> MSENQNEKVYDLSFFMPGQTI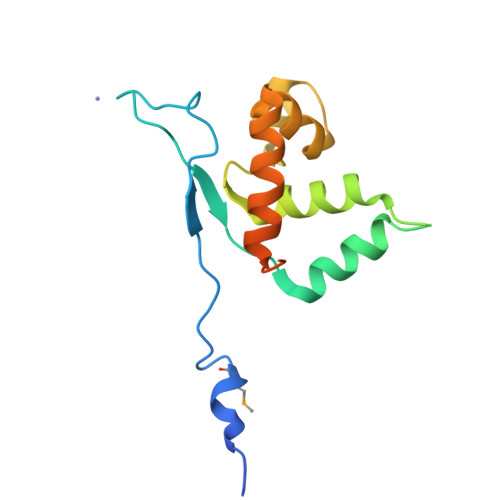DAEEVEVPISKRFVDKEGNVVPFIFKAITTDRIDELEKENTTYKNVKGRGRVKELDSQRFYARIAVETTVYPTFKAKELREAYKTEDPVEVAKRVLSVGGEYANWLNKAIEINGFDDDLEDLEEAAKNLEHHHHHH4-ethylmorpholine 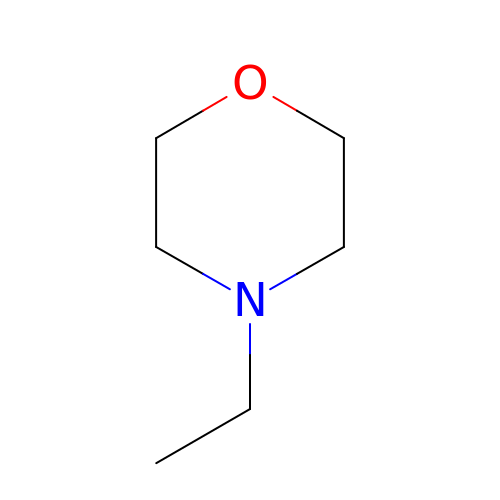| C6 H13 N O | HVCNXQOWACZAFN-UHFFFAOYSA-N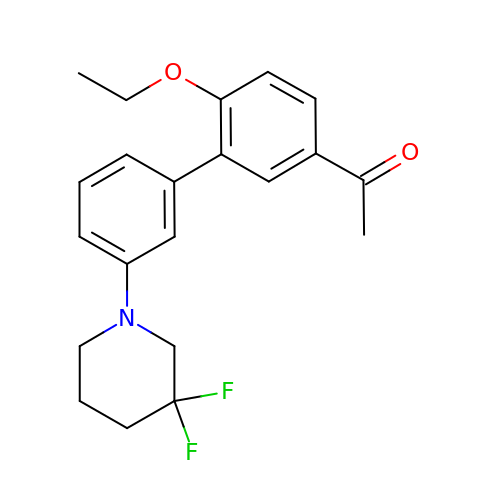1-[3-[3-[3,3-bis(fluoranyl)piperidin-1-yl]phenyl]-4-ethoxy-phenyl]ethanone | C21 H23 F2 N O2 | SEPRJZNGZUHEJW-UHFFFAOYSA-N>[2x]TGCVLNKLFQLPTPPLSRHQLKRLEEHRYQSAGRSLLEPLMQGYWEWLVRRVPSWIAPNLITIIGLSINICTTILLVFYCPTATEQAPLWAYIACACGLFIYQSLDAIDGKQARRTNSSSPLGELFDHGCDSLSTVFVVLGTCIAVQLGTNPDWMFFCCFAGTFMFYCAHWQTYVSGTLRFGIIDVTEVQIFII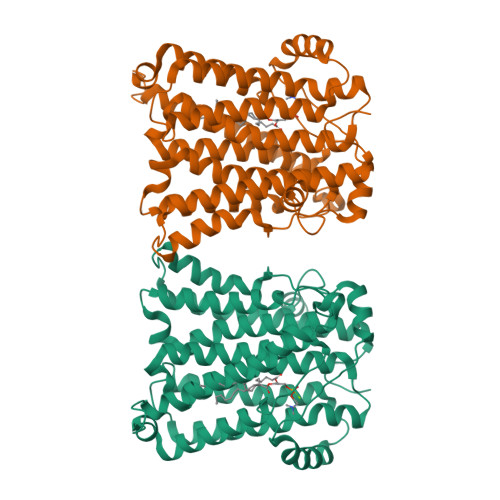IMHLLAVIGGPPFWQSMIPVLNIQMKIFPALCTVAGTIFSCTNYFRVIFTGGVGKNGSTIAGTSVLSPFLHIGSVITLAAMIYKKSAVQLFEKHPCLYILTFGFVSAKITNKLVVAHMTKSEMHLHDTAFIGPALLFLDQYFNSFIDEYIVLWIALVFSFFDLIRYCVSVCNQIASHLHIHVFRIK>GYTLWNDQIVKDEEVKIDKEDRGYQFGDGVYEVVKVYNGEMFTVNEHIDRLYASAEKIRITIPYTKDKFHQLLHELVEKNELNTGHIYFQVTRGTSPRAHQFPENTVKPVIIGYTKENPR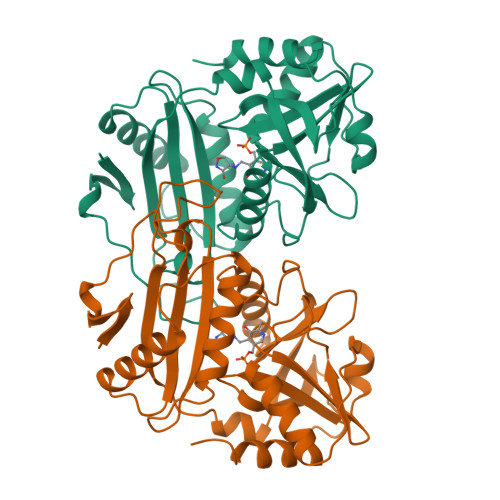PLENLEKGVKATFVEDIRWLRCDIKSLNLLGAVLAKQEAHEKGCYEAILHRNNTVTEGSSSNVFGIKDGILYTHPANNMILKGITRDVVIACANEINMPVKEIPFTTHEALKMDELFVTSTTSEITPVIEIDGKLIRDGKVGEWTRKLQKQFETKIPKPLHI[2x]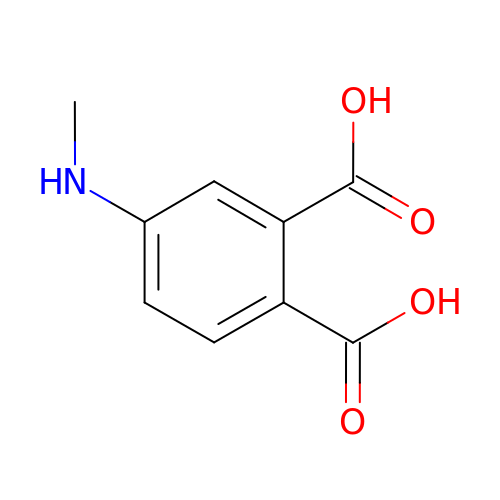4-(methylamino)benzene-1,2-dicarboxylic acid | C9 H9 N O4 | WIVUEBNYALSDOC-UHFFFAOYSA-N>[4x]GSYDSSSS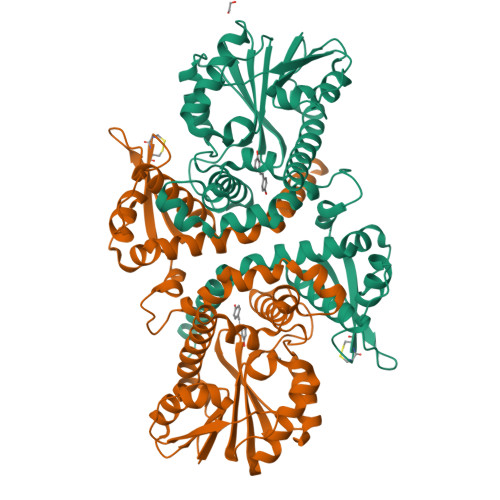SSNDSSARNEEDESCMFALKLLGGFAVPFTIKAVIELGVMDQLLTAERAMSAEELVAAAVAAQLPRPEVACTMVDRLLRFLASHSVVRCTTEVVVGTDDATTTTCCRRSYAASPVCKWFARNGVEDSVLPLGMMILNKTFLDSWQNITDAVLEGAAPFEKTYGMPMFEYLSTNGPLNTVFHEAMANHSMIITKKLLKFFRGFEGLDVLVDVGGGNGTTLQMIRGQYKNMRGINYDLPHVIAQAAPVEGVEHVGGSMFDNIPRGNAVLLKWILHDWDDKACIKILKNCYTALHVRGKVIVLEYVVPDEPEPTLAAQGAFELDLTMLVTFGSGKERTQREFSELAMEAGFSREFKATYIFANVWALEFTK>[2x]AQIDLNITCRFAGVFHVEKNGRYSISRTEA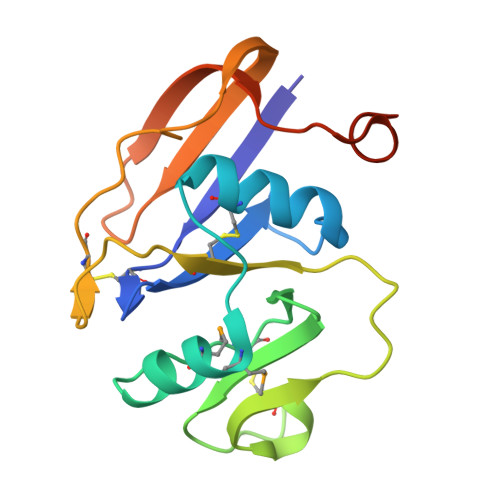ADLCKAFNSTLPTMAQMEKALSIGFETCRYGFIEGHVVIPRIHPNSICAANNTGVYILTSNTSQYDTYCFNASAPPEEDCTSVTDLPNAFDGPITITIVNRDGTRYVQKGEYRTNPEDIYPSNPTDDDV3-(3-fluorophenyl)-N-{[2-(1H-imidazol-1-yl)pyrimidin-4-yl]methyl}propan-1-amine 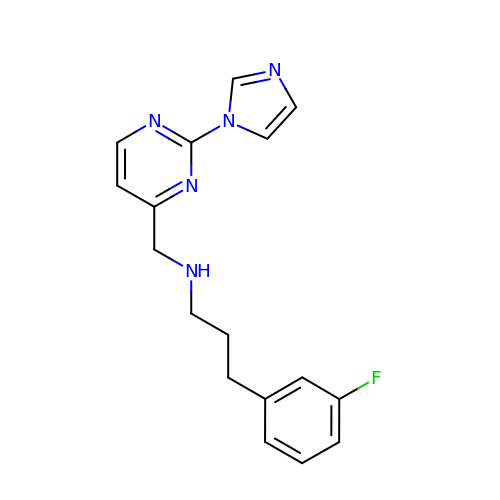| C17 H18 F N5 | MFPWDFATUAKLEA-UHFFFAOYSA-N> GMNLDSYERTGLRVSLDLVNIATPGSRRG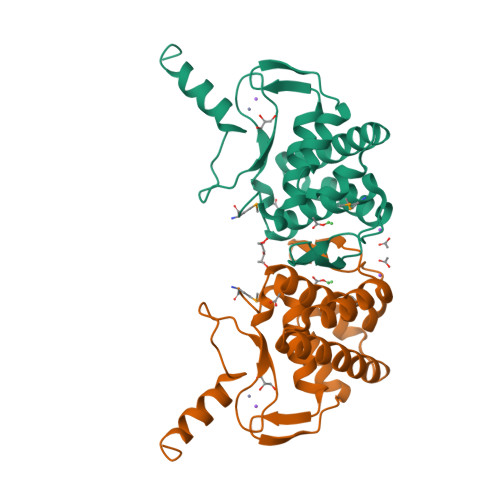TPHTGGCVIEDLHDLLKDDPASVAQLGDDHVEGFVELARLLHTAIDALSNGQVATAATALNHLLRKHPATPELAQDPDGTWRLHHHPLDAELVPMWTAICAEGLAREIGHQNVRRFGICNAHRCDRVYFDTSRNGTRQYCSLACQNRVKAAAFRERRAT>[2x]SATNGKLFPWAQIRLPTAVVPLRYELSLHPNLTSMTFRGSVTISVQALQVTWNIILHSTGHNISRVTFMSAVSSQEKQAEILEYAYHGQIAIVAPEALLAGHNYTLKIEYSANISSSYYGFYGFSYTDESNEKKYFAATQFEPLAARSAFPCFDEPAFKATFIIKIIRDEQYTALSNMPKKSSVVLDDGLVQDEFSESVKMSTYLVAFIVGEMKNLSQDVNGTLVSIYAVPEKIGQVHYALETTVKLLEFFQNYFEIQYPLKKLDLVAIPDFEAGAMENWGLLTFREETLLYDSNTSSMADRKLVTKII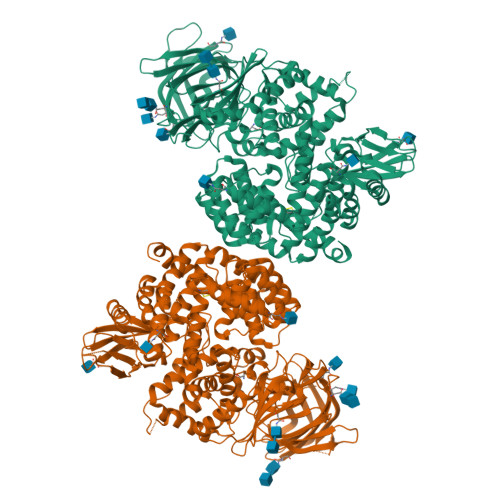AHELAHQWFGNLVTMKWWNDLWLNEGFATFMEYFSLEKIFKELSSYEDFLDARFKTMKKDSLNSSHPISSSVQSSEQIEEMFDSLSYFKGSSLLLMLKTYLSEDVFQHAVVLYLHNHSYASIQSDDLWDSFNEVTNQTLDVKRMMKTWTLQKGFPLVTVQKKGKELFIQQERFFLNMKPEIQPSDTSYLWHIPLSYVTEGRNYSKYQSVSLLDKKSGVINLTEEVLWVKVNINMNGYYIVHYADDDWEALIHQLKINPYVLSDKDRANLINNIFELAGLGKVPLKRAFDLINYLGNENHTAPITEALFQTDLIYNLLEKLGYMDLASRLVTRVFKLLQNQIQQQTWTDEGTPSMRELRSALLEFACTHNLGNCSTTAMKLFDDWMASNGTQSLPTDVMTTVFKVGAKTDKGWSFLLGKYISIGSEAEKNKILEALASSEDVRKLYWLMKSSLNGDNFRTQKLSFIIRTVGRHFPGHLLAWDFVKENWNKLVQKFPLGSYTIQNIVAGSTYLFSTKTHLSEVQAFFENQSEATFRLRCVQEALEVIQLNIQWMEKNLKSLTWWL There are three parts to the flagellar structure: the trans-membrane basal body that functions as the motor, the connecting rod and hook, and the flagellar filament that acts like a helical propeller. Our current understanding of supercoiling in bacterial flagellar filaments, referred to as polymorphic switching, is based upon the notion that protofilaments within the flagellar filament can exist in two discrete states, that differ slightly in length. The “short” state results from a protofilament having a right-handed inclination (the R-state), while the “long” state results from a protofilament having a left-handed inclination (the L-state). To reconstruct filaments at high resolution, all protofilaments must be “locked” into the same state, either L- or R-type, producing straightened filaments that lead to non-motile bacteria.

While the three L-type mutants (E115G, S285P, and S17P) have a left-handed 11-start helix, the four R-type mutants (N226Y, A233V, H84R and A39VN133H) have a right-handed 11-start helix, and the designations L and R correspond to the hand of these 11-start helices. The L-type 11-start helices are tilted left by ~ 1.7° and the R-type 11-start helices are tilted right by ~ 3.9°. In R-type subunits of B. subtilis, the side chain of E115 in S0 forms two conserved hydrogen bonds with the side chain of N240 in subunit S+5. These two sites (E115G and N240) are mostly conserved among different bacterial species, and we also detected the same interaction in the R-type A443V mutant in P. aeruginosa. In the B. subtilis E115G mutant, the filaments lose this conserved R-type interaction and therefore formed a left-handed filament.

>MRINHNIAALNTLNRLSSNNSASQKNMEKLSSGLRINRAGDDAAGLAISEKMRGQIRGLEMASKNSQDGISLIQTAEGALTETHAILQRVRELVVQAGNTGTQDKATDLQSIQDGISALTDEIDGISNRTEFNGKKLLDGTYKVDTATPANQKNLVFQIGANATQQISVNIEDMGADALGIKEADGSIAALHSVNDLDVTKFADNAADCADIGFDAQLKVVDEAINQVSSQRAKLGAVQNRLEHTINNLSASGENLTAAESRIRDVDMAKEMSEFTKNNILSQASQAMLAQANQQPQNVLQLLR[46x]Tricyclic NADPH | C21 H30 N7 O17 P3 | 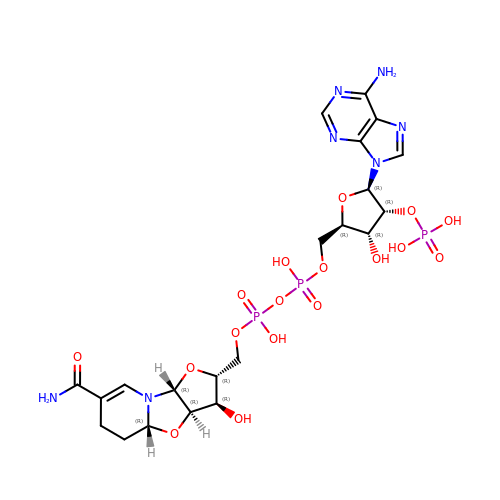AJKICLDTLPZSPE-MTKBYBFRSA-N> GSREATVLSYDGSMFMKIQLPVVMHTEAEDVSLRFRSQRAYGILMATTSRDSADTLRLELDAGRVKLTVNLGKGPETLFAGYNLNDNEWHTVRVVRRGKSLKLTVDDQQAMTGQMAGDHTRLEFHNIETGIITERRYLSSVPSNFIGHLQSLTFNGMAYIDLCKN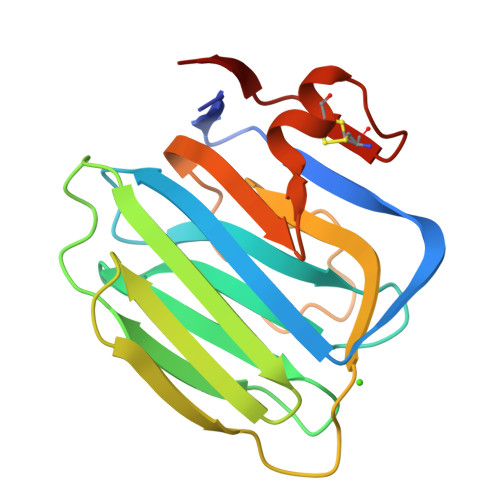GDIDYCELNARFGFRNI> G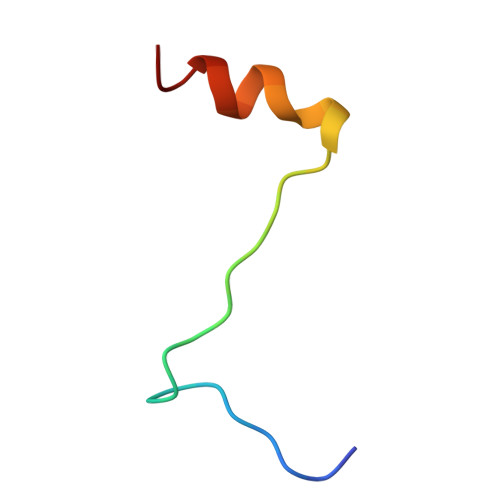GGGGGGGAASHQRVTPDWMLPLILGLYG>VRRQSRPVADGMVELPFITPKPEDELLIDPEKKRKPGVAAPQLVAGDIVAEQYEVLGVIAHGGMGWIYLANDRNVSGRIVVLKGMMAQSSVQDQGTAEAEREFLADITH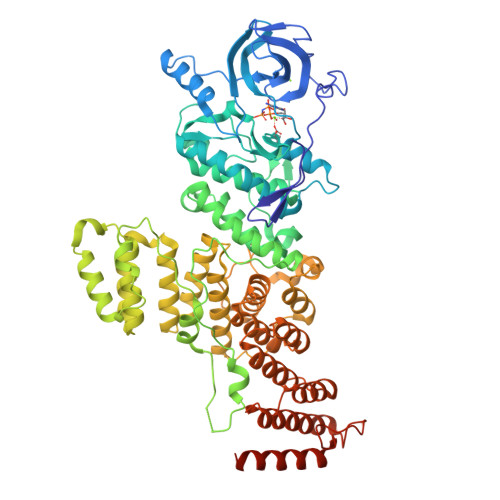PGIVKAYNFIDDPRVPGGFIVMEYVNGPSLKDRCKAQPDGVLRVDLAIGYILELLPAMDYLHQRGVVYNDLKPENVIATEDQVKLIDLGAVTGIGAFGYIYGTKGFQAPEVATHGPSISSDIFTIGRTLAALTMPLPVEDGVLAPGIPSPKNSPLLRRHLSFYRLLQRATADDPQHRFRNVSELRTQLYGVLREILAVRDGKQYPPQHSLFSPQRSTFGTKHLVFRTDRIIDGIERQARITAPEIVSALPVPLIDRTDPGARMLSGSSYAEPSETLETLRNSMEDEQYRQSIEIPLGVVRALLDLGFTTEARQWLETLEGRIGDDWRHKWFSGITYLLLDDYATAQVFFNHVLTILPGEAAPKLALAAVDELILQQIGAESTAYLTPDIVSATATLSKDFEDLDASAFESLSDTWSHISSDPHVVRFHSLRLYALVWATNPTTVSSAFGLARQLMAENQIELAVQALDKLPQSSTHYRMATLTTILLLVSSNLSESRIRRAARRLTEIPTNEPRFNQIKIAIMSAGLSWLRERKLKASASANPLFEYPFSQKGLRTGISEALRIQARSAPFPHHRYALVDMANAVRPLSWF[2x]> GMADTLERVTKIIVDRLGVDEADVKLEASFKEDLGADSLDVVELVMELEDEFDMEISDEDAEKIATVGDAVN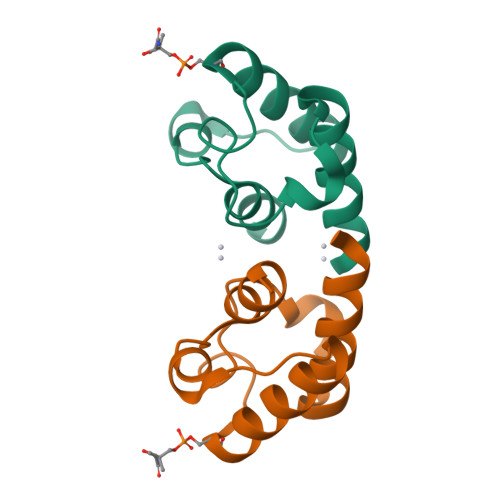YIQNQQ Leucine-rich repeat kinase 2 (LRRK2) is a highly pursued drug target for Parkinson’s disease (PD), which is the second most common neurodegenerative disease projected to affect 17.5 million people by 20401. LRRK2 is a 286-kDa protein containing seven domains (ARM, ANK, LRR, ROC, COR, KIN, and WD40) with kinase and GTPase activities. Autosomal dominant LRRK2 mutations with higher kinase activity are leading genetic causes of both familial and sporadic late-onset PD cases. Here we report high-resolution cryo-EM structures of LRRK2 in complex with a panel of small molecules, including two type I (LRRK2-IN-1 and GNE-7915) and three type II inhibitors (rebastinib, ponatinib, and GZD-824).

For type I inhibitors, we designed an LRRK2RCKW construct with M1732R mutation (LRRK2RCKWm) based on the following observations and rationales. Therefore, we introduced the M1732R mutation, which disrupts COR-B dimerization and LRRK2 filamentation, to prevent protein aggregation. Second, the binding of type I inhibitors could lead to a kinase-closed active-like conformation with flexible N-terminal ARM-ANK-LRR domains, which did not show interaction with the rest of the protein upon activation. We determined LRRK2RCKWm structures with LRRK2-IN-1 and GNE-7915 at overall resolutions of 3.5 and 3.8 Å, respectively. In our structures, type I inhibitors display well-resolved cryo-EM densities, which allow the analyses of protein–inhibitor interactions in atomic details and comparison with ATP binding in the active state. Despite small differences in the overall structures, LRRK2 KIN domains with type I inhibitors and ATP are almost identical with RMSD < 0.5 Å. To understand what contributes to the selectivity of GNE-7915 and LRRK2-IN-1 for LRRK2, we compare LRRK2 and its homologous structures with type I inhibitors bound. LRRK2 with type 1 inhibitors bound show conformational differences compared to the active LRRK2cent protomer in the Rab29–LRRK2 complex with a small rotational movement of ROC-COR domains. The differences likely result from the tetramerization of LRRK2 in the Rab29–LRRK2 complex, where ROC-COR domains play a key role in mediating LRRK2 oligomerization.

> KKAVPYNRMKLMIVGNTGSGKTTLLQQLMKTKKSDLGMQSATVGIDVKDWPIQIRDKRKRDLVLNVWDFAGREEFYSTHPHFMTQRALYLAVYDLSKGQAEVDAMKPWLFNIKARASSSPVILVGTHLDVSDEKQRKACMSKITKELLNKRGFPAIRDYHFVNATEESDALAKLRKTIINESLNFKIRDQLVVGQLIPDCYVELEKIILSERKNVPIEFPVIDRKRLLQLVRENQLQLDENELPHAVHFLNESGVLLHFQDPALQLSDLYFVEPKWLCKIMAQILTVKVEGCPKHPKGIISRRDVEKFLSKKRKFPKNYMTQYFKLLEKFQIALPIGEEYLLVPSSLSDHRPVIELPHCENSEIIIRLYEMPYFPMGFWSRLINRLLEISPYMLSGRERALRPNRRYWRQGIYLNWSPEAYCLVGSEVLDNHPESFLKITVPSCRKGCILLGQVVDHIDSLMEEWFPGLLEIDICGEGETLLKKWALYSFNDGEEHQKILLDDLMKKAEEGDLLVNPDQPRLTIPISQIAPDLILADLPRNIMLNNDELEFEQAPEFLLGDGSFGSVYRAAYEGEEVAVKIFNKHTSLRLLRQELVVLCHLHHPSLISLLAAGIRPRMLVMELASKGSLDRLLQQDKASLTRTLQHRIALHVADGLRYLHSAMIIYRDLKPHNVLLFTLYPNAAIIAKIADYGIAQYCCRMGIKTSEGTPGFRAPEVARGNVIYNQQADVYSFGLLLYDILTTGGRIVEGLKFPNEFDELEIQGKLPDPVKEYGCAPWPMVEKLIKQCLKENPQERPTSAQVFDILNSAELVCLTRRILLPKNVIVECMVATHHNSRNASIWLGCGHTDRGQLSFLDLNTEGYTSEEVADSRILCLALVHLPVEKESWIVSGTQSGTLLVINTEDGKKRHTLEKMTDSVTCLYCNSFSKQSKQKNFLLVGTADGKLAIFEDKTVKLKGAAPLKILNIGNVSTPLMCLSESTNSTERNVMWGGCGTKIFSFSNDFTIQKLIETRTSQLFSYAAFSDSNIITVVVDTALYIAKQNSPVVEVWDKKTEKLCGLIDCVHFLREVTVKENKESKHKTSYSGRVKTLCLQKNTALWIGTGGGHILLLDLSTRRLIRVIYNFCNSVRVMMTAQLGSLKNVMLVLGYNRKNTEGTQKQKEIQSCLTVWDINLPHEVQNLEKHIEVRKELAEKMRRTSVE>[6x]SFSMVTRYAHSPEDIQHYDTSKLRHEFLMEKIFNPGDILLTYTYNDRMIFGGVMPTDEPLEIKLSTELGVDFFLQRRELGIINIGGAGAITIDGRKDAMSNQDGYYIGMGTQKVVFTSEDRDHPA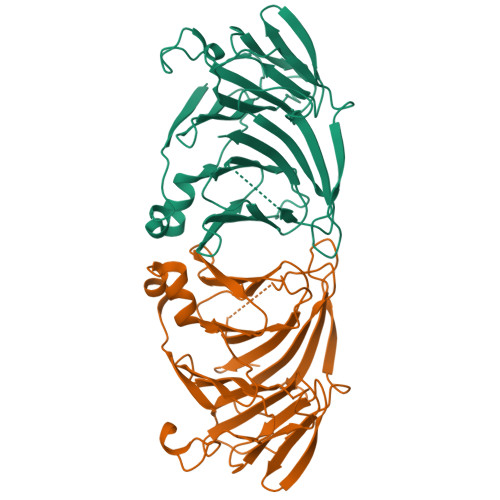KFYVVSTPAHKTYPNKKLPFATALAKPMGDQQHLNKRTIYKYIDASQMDTCQLQMGYTVLEPGSSWNTMPAHTHARRMETYMYFNFADPETRVFHFLGKPDETRHITLFNEQAVVNPSWSIHCGVGTTNYAFIWAMCGENQ> SNAQTAFWKSLLKGPPPPPNCKGHSEPCVLRTVKKAGPNCGRQFYVCARPEGHSSN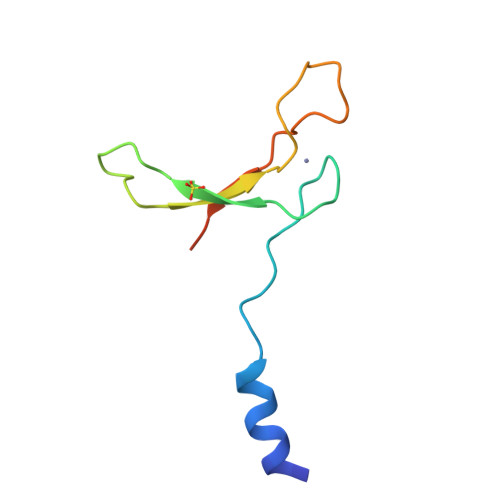PQARCNFFLWLTKKAGCED> QKEGVLRVITRNSPATYFQDRNGETGFEYELAKRFAERLGVELKIETADNLDDLYAQLSREGGPALAAAGLTPGREDDASVRYSHTYLDVTPQIIYRNGQQR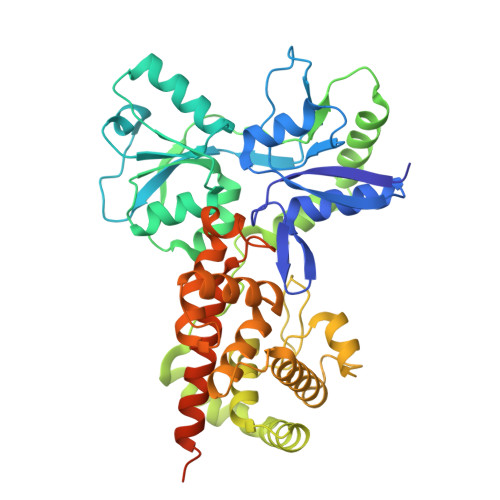PTRPEDLVGKRIMVLKGSSHAEQLAELKKQYPELKYEESDAVEVVDLLRMVDVGDIDLTLVDSNELAMNQVYFPNVRVAFDFGEARGLAWALPGGDDDSLMNEVNAFLDQAKKEGLLQRLKDRYYGHVDVLGYVGAYTFAQHLQQRLPRYESHFKQSGKQKDTDWRLLAAIGYQESLWQPGATSKTGVRGLMMLTNRTAQAMGVSNRLDPKQSIQGGSKYFVQIRSELPESIKEPDRSWFALAAYNIGGAHLEDARKMAEKEGLNPNKWLDVKKMLPRLAQKQWYAKTRYGYARGGETVHFVQNVRRYYDILTWVTQPQMEGSQIAESGLHLPGVNKTRPEEDSGDEKL>[2x]RECKTESN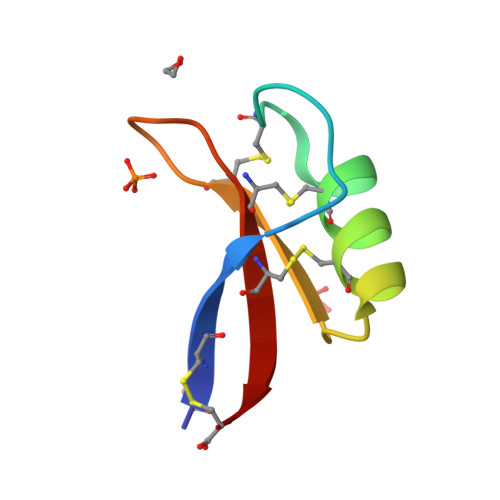TFPGICITKPPCRKACISEKFTDGHCSKILRRCLCTKPC> QGRGCLLKEIHLNVTD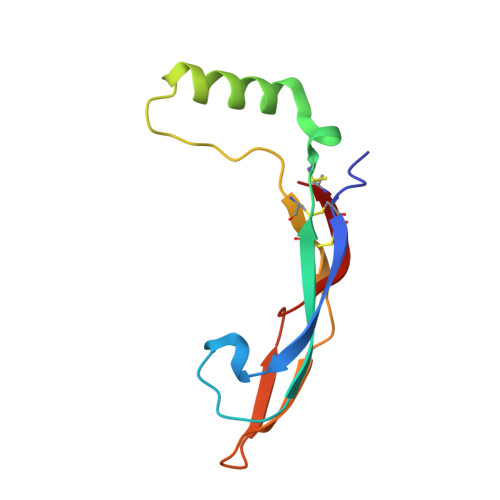LDLGYRTKEELIFRYCSGPCHDAETNYDKILNNLTHNKKLDKDTPSRTCCRPIAFDDDISFLDDSLEYHTLKKHSAKKCACV> MPSFNPVRFLELPIDIRKEVYFHLDGNFCGAHPYPIDILYKSNDVELPGKPSYKRSKRSKKLLRYMYPVFATYLNIFEYSPQLIEKWLEYAFWLRYDCLVLDCFKVNHLYDGTLIDALEWTYLDNELRLAYFNKASMLEVWYTFKEYKKWVIDSVAFDELDLLNVSNIQFNI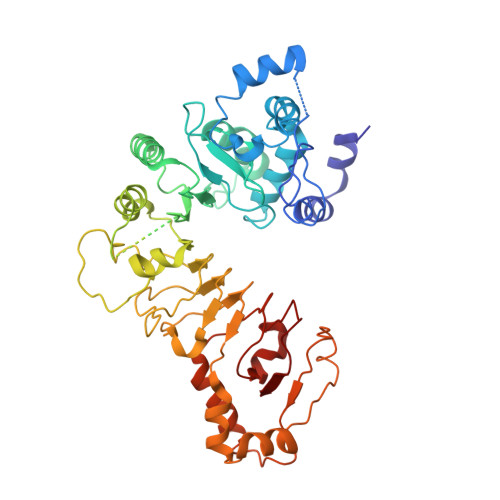DNLTPQLVDKCLSILEQKDLFATIGEVQFGQDEEVGEEKDVDVSGANSDENSSPSSTIKNKKRSASKRSHSDNGNVGATHNQLTSISVIRTIRSMESMKSLRKITVRGEKLYELLINFHGFRDNPGKTISYIVKRRINEIRLSRMNQISRTGLADFTRWDNLQKLVLSRVAYIDLNSIVFPKNFKSLTMKRVSKIKWWNIEENILKELKVDKRTFKSLYIKEDDSKFTKFFNLRHTRIKELDKSEINQITYLRCQAIVWLSFRTLNHIKLQNVSEVFNNIIVPRALFDSKRVEIYRCEKISQVLVI> MSKATEQNDKLKRAIIISAVLHVILFAALIWSSFDENIEASAGGGGGSSIDAVMVDSGAVVEQYKRMQSQESSAKRSDEQRKMKEQQAAEELREKQAAEQERLKQLEKERLAAQEQKKQAEEAAKQAELKQKQAEEAAAKAAADAKAKAEADAKAAE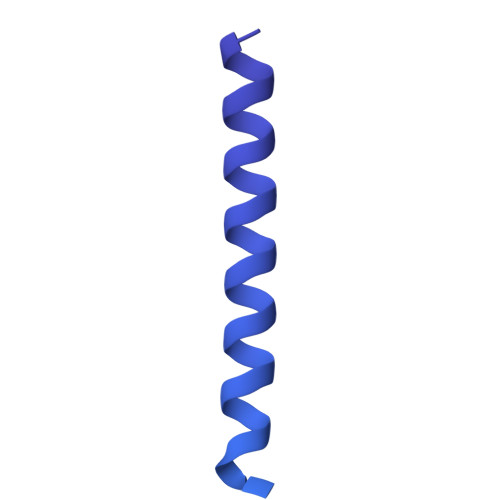EAAKKAAADAKKKAEAEAAKAAAEAQKKAEAAAAALKKKAEAAEAAAAEARKKAATEAAEKAKAEAEKKAAAEKAAADKKAAAEKAAADKKAAEKAAAEKAAADKKAAAEKAAADKKAAAAKAAAEKAAAAKAAAEADDIFGELSSGKNAPKTGGGAKGNNASPAGSGNTKNNGASGADINNYAGQIKSAIESKFYDASSYAGKTCTLRIKLAPDGMLLDIKPEGGDPALCQAALAAAKLAKIPKPPSQAVYEVFKNAPLDFKP>[2x]GAMEEKYLPELMAEKDSLDPSFTHALRLVNQEIEKFQKGEGKDEEKYIDVVINKNMKLGQKVLIPVKQFPKFNF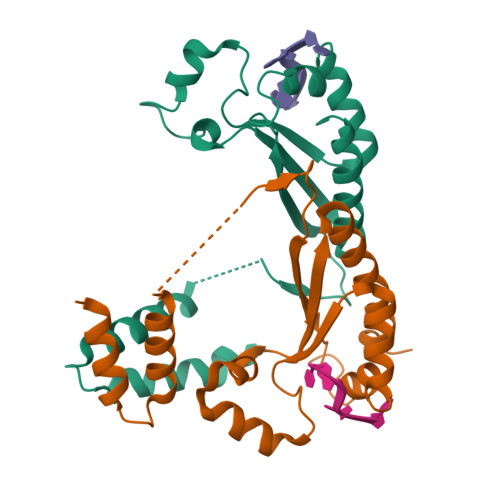VGKLLGPRGNSLKRLQEETLTKMSILGKGSMRDKAKEEELRKSGEAKYFHLNDDLHVLIEVFAPPAEAYARMGHALEEIKKFLIPDYN>GTMSSGDFGNPLRKFKLVFLGEQSVGKTSLITRFMYDSFDNTYQATIGIDFLSKTMYLEDRTVRLQLWDTAGQERFRSLIPSYIRDSTVAVVVYDITNTNSFHQTSKWIDDVRTERGSDVIIMLVGNKTDLSDKRQVSTEEGERKAKELNVMFIETSAKAGYNVKQLF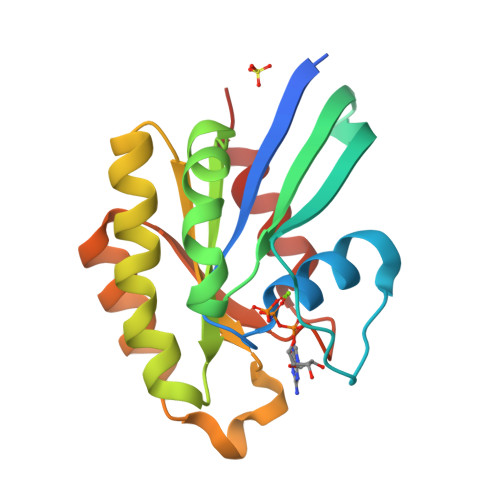RRVAAALPGMD[2x]> MTAPADTVHPAGQPDYVAQVATVPFRLGRPEELPGTLDELRAAVSARAGEAVRGLNRPGARTDLAALLAATERTRAALAPVGAGPVGDDPSESEANRDNDLAFGIVRTRGPVAELLVDAALAALAGILEVAVDRGSDLEDAAWQRFIGGFDALLGWLADPHSAPRPATVPGAGPAGPPVHQDALRRWVRGHHVFMVL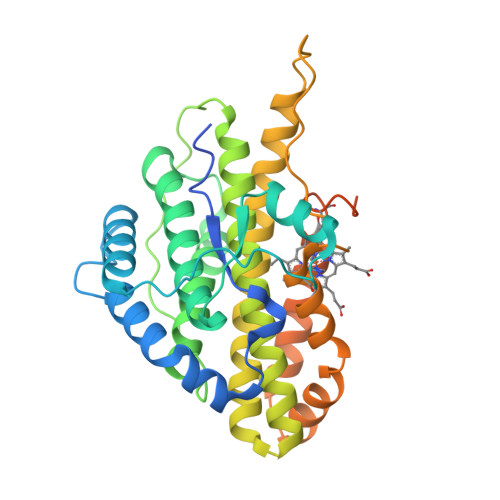AQGCALATACLRDSAARGDLPGAEASAAAAEALMRGCQGALLYAGDANREQYNEQIRPTLMPPVAPPKMSGLHWRDHEVLIKELAGSRDAWEWLSAQGSERPATFRAALAETYDSHIGVCGHFVGDQSPSLLAAQGSTRSAVGVIGQFRKIRLSALPEQPATQQGEPS>[2x]MVPISPIETVPVKLKPGMDGPKVKQWPLTEEKIKALVEICTEMEKEGKISKIGPENPYNTPVFAIKKKDSTKWRKLVDFRELNKRTQDFWEVQLGIPHPAGLKQKKSVTVLDVGDAYFSVPLDKDFRKYTAFTIPSINNETPGIRYQYNVLPMGWKGSPAIFQSSMTKILEPFRKQNPDIVIYQYMDDLYVGSDLEIGQHRTKIEELRQHLLRWGFTTPDKKHQKEPPFLWMGYELHPDKWTVQPIVLPEKDSWTVNDIQKLVGKLNWASQIYAGIKVRQLSKLLRGTKALTEVVPLTEEAELELAENREILKEPVHGVYYDPSKDLIAEIQKQGQGQWTYQIYQEPFKNLKTGKYARMKGAHTNDVKQLTEAVQKIATESIVIWGKTPKFKLPIQKETWEAWWTEYWQATWIPEWEFVNTPPLVKLWYQLEKEPIIGAETFYVDGAANRETKLGKAGYVTDRGRQKVVPLTDTTNQKTELQAIHLALQDSGLEVNIVTDSQYALGIIQAQPDKSESELVSQIIEQLIKKEKVYLAWVPAHKGIGGNEQVDKLVSAG;>MAHHHHHHALEVLFQGPISPIETVPVKLKPGMDGPKVKQWPLTEEKIKALVEICTEMEKEGKISKIGPENPYNTPVFAIKKKDSTKWRKLVDFRELNKRTQDFWEVQLGIPHPAGLKQKKSVTVLDVGDAYFSVPLDKDFRKYTAFTIPSINNETPGIRYQYNVLPQGWKGSPAIFQSSMTKILEPFRKQNPDIVIYQYMDDLYVGSDLEIGQHRTKIEELRQHLLRWGFTTPDKKHQKEPPFLWMGYELHPDKWTVQPIVLPEKDSWTVNDIQKLVGKLNWASQIYAGIKVRQLSKLLRGTKALTEVVPLTEEAELELAENREILKEPVHGVYYDPSKDLIAEIQKQGQGQWTYQIYQEPFKNLKTGKYARMKGAHTNDVKQLTEAVQKIATESIVIWGKTPKFKLPIQKETWEAWWTEYWQATWIPEWEFVNTPPLVKLWYQ[2x]

Conceptually, HBV and HIV-1 RTs share common metal-dependent dNTP-binding and catalytic mechanism of nucleotide addition to the 3′-end of the primer DNA, whereas amino acid differences around the N-site probably result in different NRTI sensitivities. In this study, we showed that the Q151M mutation of HIV-1 RT confers high ETV and EFdA sensitivity upon HIV-1. The HIV-1 RTQ151M further enabled crystal structure analysis of HIV-1 RT in complex with ETV-TP. We also determined the crystal structure of HIV-1 RTQ151M in complex with DNA, DNA:dGTP, and DNA:ETV-TP, which revealed that ETV-TP is bound at the N-site, directly pushing the Met184 side chain.

For crystallization of the RTQ151M:DNA binary complex, the previously developed 38-mer DNA aptamer was applied, albeit with 3 base substitutions to trap guanosine analogue ETV-TP at the N-site. There are two RTQ151M heterodimers (p66/p51) in the asymmetric unit of the rhombohedral R3 lattice. The final refined model contains amino acid residues 3–553 for chains A/C (p66 subunit), 4–427 for chains B/D (p51 subunit) except 214–230 owing to poor electron density, and two DNA aptamers (nucleotides from −1 to 33 for chain E and from −4 to 33 for chain F). In the previously reported RTWT:DNA structure, the side-chain of Gln151 interacted with the adenine base of the dA0 via ordered solvent molecules, stabilizing base stacking with the cytosine base of dC127. In contrast, the present structure showed that the hydrophobic side-chain of Met151 keeps nearby residues, the base moiety of dC0, and solvent away, and that the cytosine base of dC0 is deviated by approximately 35° relative to the guanine base of dG1. Consequently, the present structure of the RTQ151M:DNA binary complex exhibits a more open conformation than that of the previously reported RTWT:DNA structure. These results indicated that the bulky, hydrophobic Met151 side-chain increases the flexibility of the N-site and forms a distinct conformational state in the absence of dNTP/NRTI. In contrast, apparent local conformational changes were observed in the β2-β3 region of the finger domain between the binary and ternary complexes with maximum atomic displacement of approximately 8.5 Å.(1R,10aS)-1,2,10,10a-tetrahydrophenazine-1-carboxylic acid | C13 H12 N2 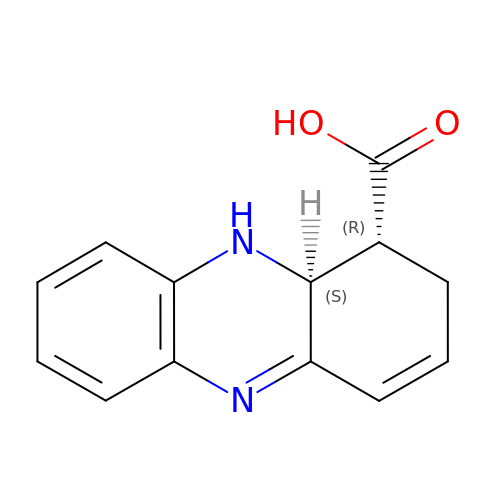O2 | JMGCBMVXHPNSFZ-PELKAZGASA-N>[2x]MFFTTPQPELSFDAMTIVGNLNKTNAKKLSDFMSTEPQIRLWDILQTKFKAKALQEKVYIEYDKVKADSWDRRNMRVEFNPNKLTHEEMLWLKQNIIDYMEDDGFTRLDLAFDFEDDLSDYYAMTDKAVKKTIFYGRNGKPETKYFGVRDSDRFIRIYNKKQERKDNADVEVMSEHLWRVEIELKRDMVDYWNDCFNDLHILKPDWSSLEKVKDQAMIYMLIHEESTWGKLERRTKNKYREMLKSISEIDLTDLMKLTLKENEKQLQKQIEFWQREFRFWE

In Gram-positive organisms, the smaller plasmids often replicate via a rolling circle mechanism, a process mediated by a multi-functional replication initiation protein (Rep) encoded on that plasmid. The Rep proteins possess two related catalytic activities, a type-I topoisomerase-like cleavage activity in which they form a nick in the (+) strand at the origin of replication to initiate DNA synthesis, and a religation activity to join the ends of the parental strand that is displaced during replication. Despite low overall sequence identity, there is a high degree of structural conservation between the catalytic domains of the Rep proteins from these Geobacillus stearothermophilus and Staphylococcus aureus plasmids. Structure-based sequence alignment reveals the conserved residues are almost exclusively located in the β-strands containing the Rep_trans motifs, and it is likely the crescent-shaped catalytic domain represents the canonical fold for the Rep_trans protein family.

In this report we describe the structure determination of the core domain of replication initiator protein of cryptic plasmid pSTK1 (25,26) from Geobacillus stearothermophilus (RepSTK1 residues 1–269 (27), hereafter referred to as RepSTK1). This was then used to aid the structure solution of two staphylococcal Rep variants, RepDE and RepDN (containing the 21 kDa fragment of RepD fused to the 14 kDa fragment of RepE or RepN, respectively). Constructs of RepDE and RepDN spanning residues 35–314 were used for crystallisation studies, since the first 34 amino acids are predicted to be disordered and had previously been shown to be dispensable for protein function. RepDE crystallized in space group C2, but all attempts to generate experimental phases were unsuccessful. Crystals of both RepDE and RepDN contain two molecules per asymmetric unit as a non-crystallographic dimer and the final structural model spans residues 39–308 for all subunits. The catalytic residues of RepDE are found in the crescent shaped domain, within a 10-stranded β-sheet, the outer surface of which is decorated with 7 α-helices. In this protein the catalytic domains do not form a closed ring, but rather a ‘horseshoe’ where they are rotated by 15° relative to their position in RepSTK1. RepDE and RepDN also contain an additional all-helical domain (helices α6–α9, residues 237–280) previously identified to contain the residues responsible for recognition of the ICRIII sequence at the origin of replication, conferring specificity between the protein and its plasmid substrate. Comparison of the active sites of RepDE and RepSTK1 show that they are remarkably similar and can be superposed with an r.m.s.d. of 0.4 Å between the Cα positions of the catalytic residues. Mapping these residues onto the RepDE structure identifies a potential interaction interface for PcrA helicase, at the open end of the catalytic domain.>[2x]MNVMRHSWLAVAGIAGLLAFPPVDACTLWGAAGTASMEGSLLAKNRDWKPDHAQSLRLLHPEH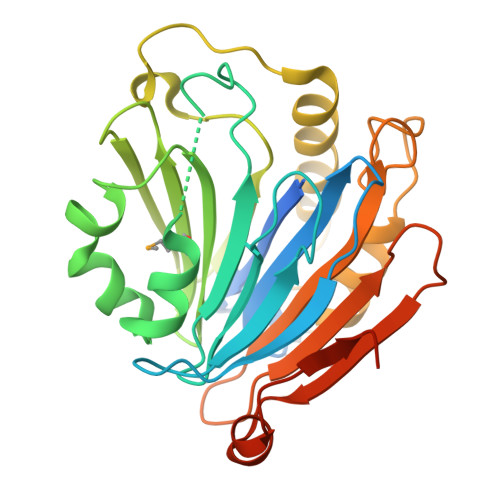GYAYLGLYADNGSEPGIKAGVNQKGLAVVAAEASSLPRALRADSARHGVLTRLLRDYGSLDEVASAADKLFAQARPVFLLLADAGGLMQVEIGQHGRYRLIRQQSGTLAHTNHYADTSLLDGAQTIGPSSQARLERIRFLLDQHPAHTLSEFERLSRDRHDGPDNSLWRSGREHTLAGWRIALPAGAPPRLQLTLANPGRAERDGDYALDSAFWAQPARTLLPKLAAALEHHHHHH> MTTVNSNINVDADFNELPFQAVKYIQKIKPGFKPQIAFILGSGLGDLVDQITNDTTISYADIPGFPVSSVHGHAGELVLGDLCGVPVMCMKGRGHFYEGKGMSIMTNPVRTFKLMGCEFLFCTNAAGSLRPEVLPGSVVMLKDHI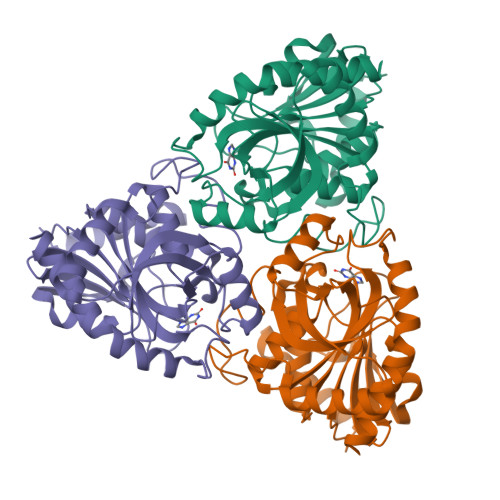NTMPGTPLVGPNDDRFGPRFFSLANAYDKDLRADMAKIAQQLDIPLTEGVFVSYPGPCFETPAEIRMMQIIGGDVVGMSVVPEVLSAAHCGLKVIALTAITNLAEGLSDVVLSHEQTLKFAKVASVNFTKLIEAFLKSKALR> MTADRPALRTGDRDTRLSFGSNLSSFTDYLRGHAPELLPENRIGHRSHSTRGGDGMESGDLAPHGTTIVALTYKGGVLLAGDRRATQGNLIASRDVEAVYVTDEYSAAGIAGTAGIAIELVRLFAVELEHYEKIEGVPLTFDGKANRLASMVRGNLGAAMQGLAVVPLLVGYDLDADDESRAGRIVSYDVVGGRYEERAGYHAVGSGSLFAKSALKKIYSPDSDEETALRAAIESLYDAADDDSATGGPDLTRGIYPTAVTITQAGAVHVSEETTSE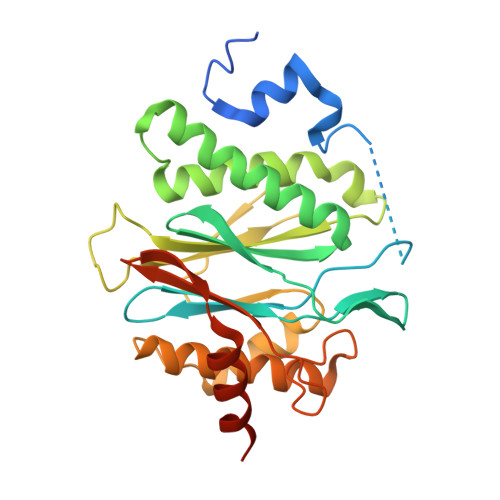LARRIVAERTEQGGSAR> DLADRFAELERRYDA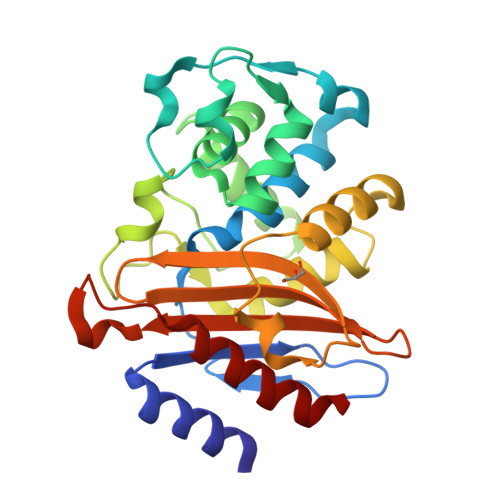RLGVYVPATGTTAAIEYRADERFAFCSTFKAPLVAAVLHQNPLTHLDKLITYTSDDIRSISPVAQQHVQTGMTIGQLCDAAIRYSDGTAANLLLADLGGPGGGTAAFTGYLRSLGDTVSRLDAEEPELNRDPPGDERDTTTPHAIALVLQQLVLGNALPPDKRALLTDWMARNTTGAKRIRAGFPADWKVIDKTGTGDYGRANDIAVVWSPTGVPYVVAVMSDRAGGGYDAEPREALLAEAATCVAGVLA> S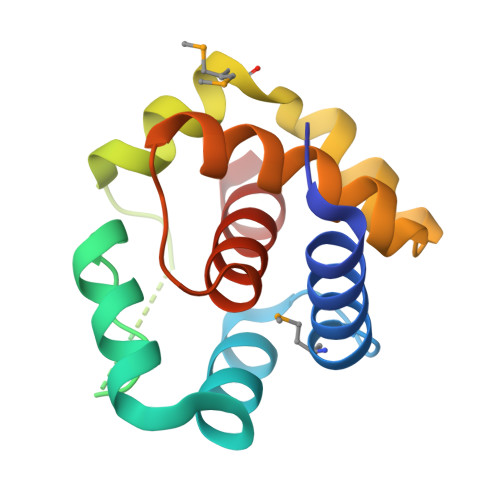DQLEDSEVEAVAKGLEEMYANGVTEDNFKNYVKNNFAQQEISSVEEELNVNISDASTVVQARFNWNALGSCVANKIKDEFFAMISISAIVKAAQKKAWKELAVTVLRFAKANGLKTNAIIVAGQLALWAVQCGLS>MAKRILCFGDSLTWGWVPVEDGAPTERFAPDVRWTGVLAQQLGADFEVIEEGLSARTTNIDDPTDPRLNGASYLPSCLATHLPLDLVIIMLGTNDTKAYFRRTPLDIALGMSVLVTQVLTSAGGVGTTYPAPKVLVVSP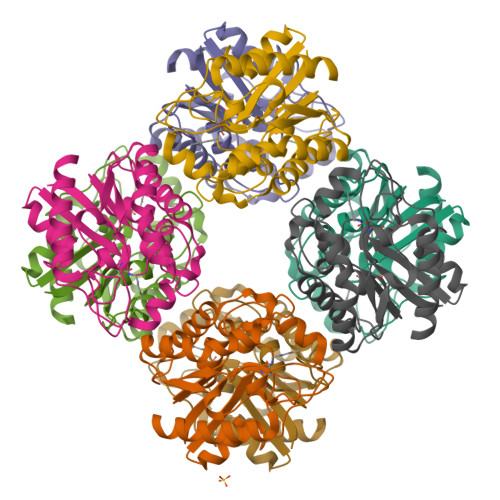PPLAPMPHPWFQLIFEGGEQKTTELARVYSALASFMKVPFFDAGSVISTDGVDGIHFTEANNRDLGVALAEQVRSLL[8x]> QDLTVKMTDLQTGKPVGTIELSQNKYGVVFIPELADLTPGIHGFHIHQNGSCASSEKDGKVVLGGAAGGHYDPEH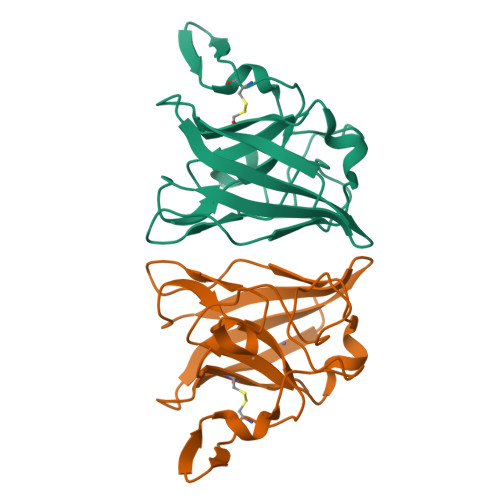TNKHGFPWTDDNHKGDLPALFVSANGLATNPVLAPRLTLKELKGHAIMIHAGGDNHSDMPKALGGGGARVACGVIQ>MANVIKARPKLYVMDNGRMRMDKNWMIAMHNPATIHNPNAQTEFVEFPIYTVLIDHPEGKILFDTSCNPNSMGPQGRWAESTQQMFPWTATEECYLHNRLEQLKVRPEDIRYVVASHLHLDHAGCLEMFTNATIIVHEDEFNGALQCYARNQKEGAYIWADIDAWIKNNLQWRTVKRHEDNILLAEGVKVLNFGSGHAWGMLGLHVELPETGGIILASD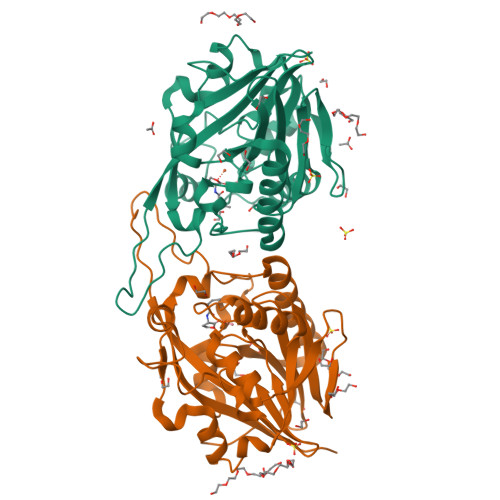AIYTAESYGPPIKPPGIIYDSLGYMNTVERIRRIAQETKSQVWFGHDAEQFKKFRKSTEGYYE[2x]> 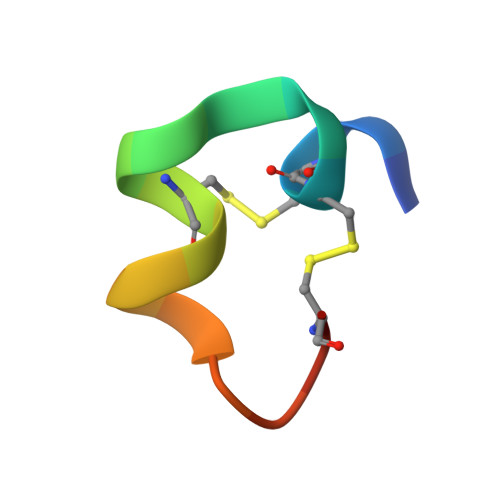SGCCSNPACRVNNPNICX>GQNHHEVVKFMDVYQRSYCHPIETLVDIFQEYPDEIEYIFKPSCVPLMRCGGCCNDEGLECVPTEESNITMQIMRIKPHQGQHIGEMSFLQHNKCECRPKKD[2x];>[2x]CAAELAALEAEL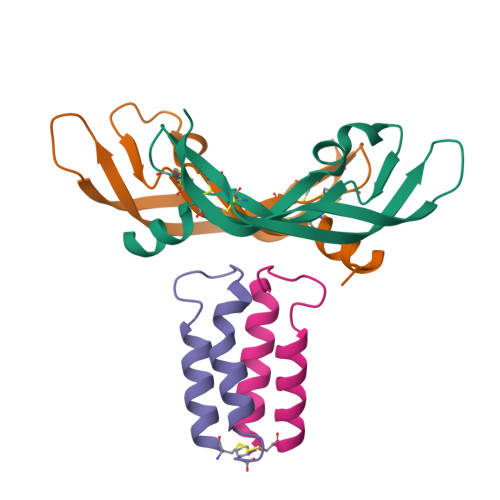AALEGPWKGYPIPYGKLQFLIKKLKQLKVAC> MSGSVSGCGSGGCSIVWFRRDLRVEDNPALAAAVRAGPVIALFVWAPEEEGHYHPGRVSRWWLKNSLAQLDSSLRSLGTCLITKRSTDSVASLLDVVKSTGASQIFFNHLYDPLSLVRDHRAKDVLTAQ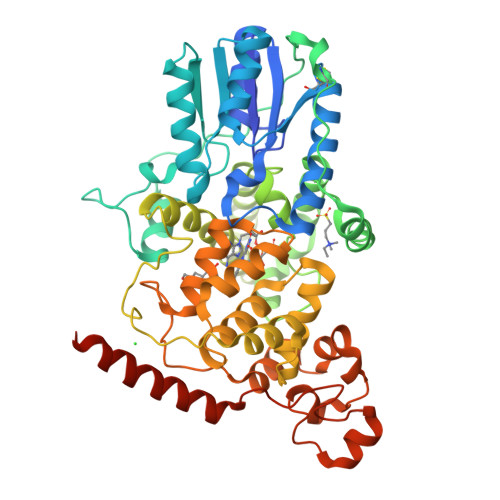GIAVRSFNADLLYEPWEVTDELGRPFSMFAAFWERCLSMPYDPESPLLPPKKIISGDVSKCVADPLVFEDDSEKGSNALLARAWSPGWSNGDKALTTFINGPLLEYSKNRRKADSATTSFLSPHLHFGEVSVRKVFHLVRIKQVAWANEGNEAGEESVNLFLKSIGLREYSRYISFNHPYSHERPLLGHLKFFPWAVDENYFKAWRQGRTGYPLVDAGMRELWATGWLHDRIRVVVSSFFVKVLQLPWRWGMKYFWDTLLDADLESDALGWQYITGTLPDSREFDRIDNPQFEGYKFDPNGEYVRRWLPELSRLPTDWIHHPWNAPESVLQAAGIELGSNYPLPIVGLDEAKARLHEALSQMWQLEAASRAAIENGSEEG Defensins are among the largest and best characterized family of cationic antimicrobial peptides (CAPs) that are produced by essentially all plant and animal species as an important component of their innate immune systems. These small (<60 amino acids), cationic, and cysteine-rich peptides can be expressed constitutively or inducibly, and exhibit broad antimicrobial activity. A key function of defensins during innate defense is their ability to permeabilize and disrupt cell membranes. Recently we demonstrated that the ability of certain plant defensins to kill fungal and tumor cells is dependent on the engagement of specific membrane phospholipids, which trigger the formation of large defensin–phospholipid oligomers.

To address this, we determined the crystal structure of a NaD1–PA complex to 2.5 Å. The structure reveals a near-flat, carpet-like oligomeric complex, which we termed the ‘membrane disruption complex’ (MDC), where a monolayer of NaD1 molecules engages PA molecules on a single side of the complex, thus mimicking the manner in which NaD1 would encounter PA molecules of target membranes. The ten dimers are arranged in a configuration that results in the formation of a mildly curved, carpet-like structure which we refer to as the membrane disruption complex (MDC), with two such 20-mers forming a large 40-meric ellipsoid complex with a total of 28 PA molecules. The MDC comprises three small arcs comprising three or four NaD1 dimers, respectively, in a 3–4–3-dimer configuration. All 14 PA binding sites identified in the MDC are identical, and are formed by residues from the signature SKILRR motif in the β2–β3 loop of NaD132. A single PA molecule makes contact with Ser35, Ile37, Leu38, and Arg40 from one NaD1 dimer, which enable Lys36 and Arg39 from a neighboring dimer to form hydrogen bonds with the phosphate head group via three water molecules that are conserved throughout the 14 PA binding sites. Intriguingly, assembly of the MDC from its constituent 3-dimer and 4-dimer arcs is achieved almost exclusively via hydrophobic interactions where Ile13 and Ile15 from the β1-α1 loop of NaD1 form continuous hydrophobic interfaces along the sides of each arc. Structure-guided mutagenesis reveals Arg39 as a key residue for the cooperative PA-mediated oligomerization and fungal growth inhibition. In contrast to wild-type NaD1 and NaD1(K36E), the NaD1(R39A) mutant lost the ability to form oligomers with PA, while still maintaining PIP2-mediated oligomerization. Since the MDC exhibits a slight curvature, we speculate that the formation of this complex is likely to induce curvature stress that would be expected to weaken the integrity of the target membrane.

>[20x]ARECKTESNTFPGICITKPPCRKACISEKFTDGHCSKILRRCLCTKPC>[4x]MKIAIPKERRPGEDRVAISPEVVKKLVGLGFEVIVEQGAGVGASITDDALTAAGATIASTAAQALSQADVVWKVQRPMTAEEGTDEVALIKEGAVLMCHLGALTNRPVVEALTKRKITAYAMELMPRISRAQSMDILSSQSNLAGYRAVIDGAYEFARAFPMMMTAAGTVPPARVLVFGVGVAGLQAIATAK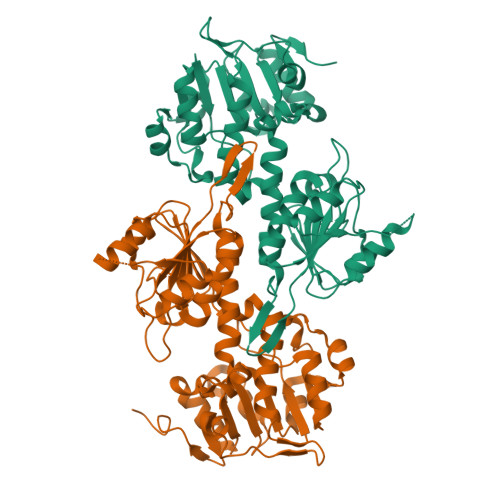RLGAVVMATDVRAATKEQVESLGGKFITVDDEAMKTAETAGGYAKEMGEEFRKKQAEAVLKELVKTDIAITTALIPGKPAPVLITEEMVTKMKPGSVIIDLAVEAGGNCPLSEPGKIVVKHGVKIVGHTNVPSRVAADASPLFAKNLLNFLTPHVDKDTKTLVMKLEDETVSGTCVTRDGAIVHPALTGQGA> NATEIRASVGKMIDGIGRFYIQMCTELKLSDYEGRLIQNSLTIERMVLSAFDTGGPIYRRVDGKWRRELILYDKEEIRRIWRQANNGDDATAGLTHMMIWHSNLNDATYQRTRALVRTGMDPRMCSLMQGSTLPRRSGAAGAAVKGVGTMVMELIRMIKRGINRRTRIAYERMCNILKGKFQTAAQRTMVDQVRESRNPGNAEFEDLIFLARSALILRGSVAHKSCLPACVYGSAVA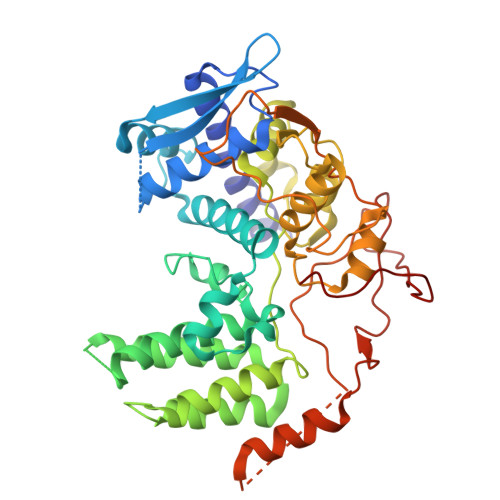SGYDFEREGYSLVGIDPFRLLQNSQVYSLIRPNENPAHKSQLVWMACHSAAFEDLRVSSFIRGTKVVPRGKLSTRGVQIASNENMETMESSTLELRSRYWAIRTRSGGNTSDMRTEIIRLMESARPEDVSFQGRGVFELSDEKATSPIVPSFDMSNEGSYFF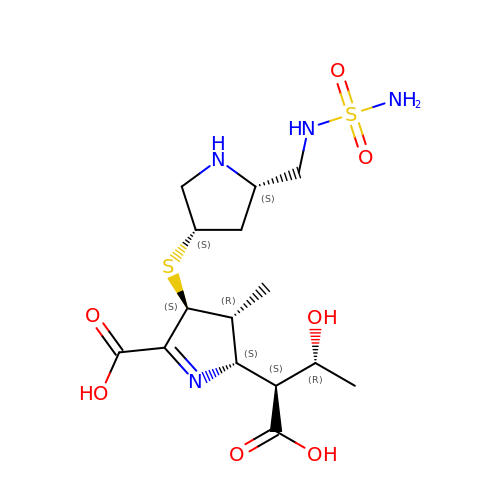(2~{S},3~{R},4~{S})-2-[(2~{S},3~{R})-1,3-bis(oxidanyl)-1-oxidanylidene-butan-2-yl]-3-methyl-4-[(3~{S},5~{S})-5-[(sulfamoylamino)methyl]pyrrolidin-3-yl]sulfanyl-3,4-dihydro-2~{H}-pyrrole-5-carboxylic acid | C15 H26 N4 O7 S2 | FODJFDYENOTZNC-UNWFBNKDSA-N>[3x]MPLDAGGQNSTQMVLAPGASIFRCRQCGQTISRRDWLLPMGGDHEHVVFNPAGMIFRVWCFSLAQGLRLIGAPSGEFSWFKGYDWTIALCGQCGSHLGWHYEGGSQPQTFFG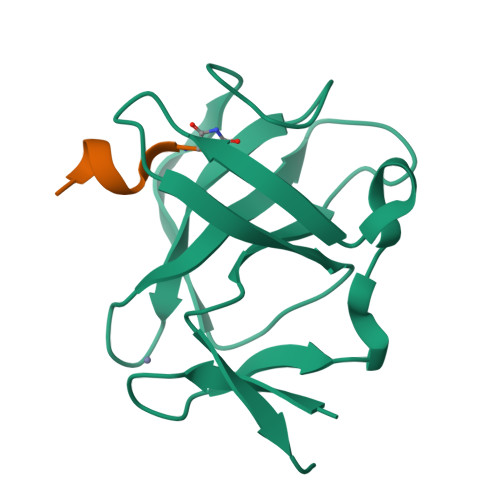LIKDRLAEGPAD;>[2x]KFFEQMQN> MHHHHHHENLYFQGAASSHKLAEANTDFAFSLYRELAKSSPDKNIFFSPVSISSALAMLSLGAKGDTHTQILEGLGFNSEADIHQGFQHLLQTLNRPKGLQLKTANGLFVDKSLKLLDSFLEDSKKLYQAEAFSVDFDPEEAKKQINDWVEKQTNGKIKDLLKDLDSDTVLVLVNAIYFKGKWKKPFDPENTKEEDFHVDEKTTVKVPMMSQKGKFYYYHDDELSCKVLELPYKGNASMLIILPDEGGLQHLEQSLTPETLSKWLKSLTRRSVELYLPKFKIEGTYDLKEVLSNLGITDLFSPGADLSGITEEKLYVS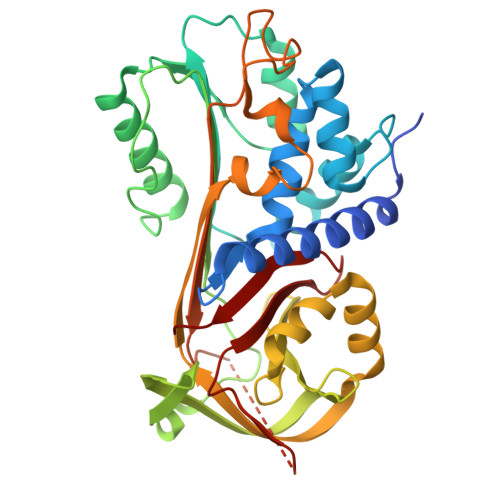KAVHKAVLEVNEEGTEAAAATFLEAIPMSIPPEFKADRPFLFLIRENKTGSILFMGKVVNP>[2x]GSH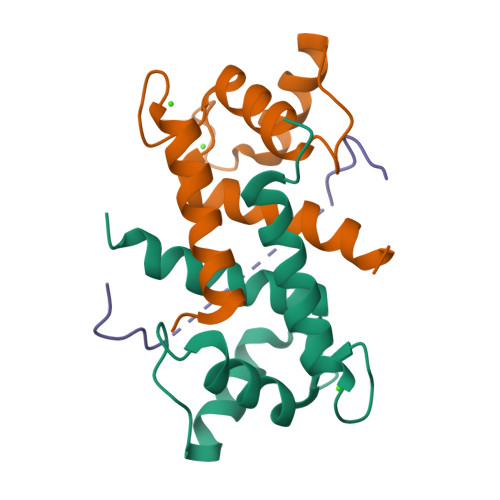MSELEKAMVALIDVFHQYSGREGDKHKLKKSELKELINNELSHFLEEIKEQEVVDKVMETLDNDGDGECDFQEFMAFVAMVTTACHEFFEHE;> GSQSQLSHQDLQLVKGAMAATYSALNSSKPTPQLKPIESSILAQRRVRKLPSTTL>MVIDSKQDLPQYTKDSGSESDSDSSNNFIVESPSIPSSKSATVVLNSEEYEDDEGDDLNGLDAELIDNITYEGDEDETMFVGLKEKQKLHLSGVFRLQVVKGGIVYNNVHYNASREILTFWHPLSQSIPTIDFSHFAGWQDTFFMPRNNRFKIRDEEFKSFPCVLRVFNSNHTGLLEAGHLYRDVNYLWKPKEPYFPLNERTTYHLLHESDRIQSLSVPGYWSTPLEKLYLSHKNAAYDTRIMVIGGKNSGKSTFLRLLLEKFTQDIRDSTTSQEELVYLDLDPGQPEYSLPDSISLNKILSSPISLGQHLCQ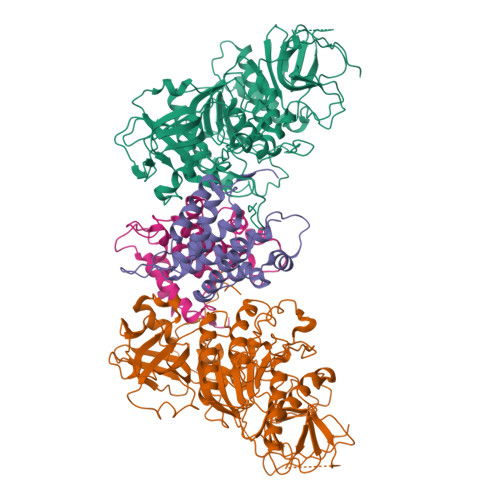GSNFQTLLQFYAGSSSPQDEPTSYLNCADKLIDHLEEQAFFGTSLLNLPGWIKGFGMQILNHIIRKYKPTHLLFLETANSKRHLDELTIPQSFSTSLRDAYAPEVVRVPAHSLNHTLSSRFHASQLRTFKILALFHKITQFDYDFAPLLKSAPLQISYGKGKSGIKGIQFPMEFQDLNPQDIKSALEGTVIGIYTYSGEDSLEVKSLNTFPILQSCTSSSKNFITLGLIHSIDTSQQIMNIYVPPCHTQILDKQPEDAQWIIVRNKTETPFCDFLPSPRTITWDDNIQIPFATFERRKKLEHVWKVRKNVMRRGQFMKR[2x];>[2x]MIPPRIVPWRDFAELEELKLWFYPKSKGTIEDKRQRAVQRVQSYRLKGSQYLPHVVDSTAQITCAVLLDEKEACLGVHQDSIPIRLSYVMALIRFVNGLLDPTQQSQFAIPLHTLAAKIGLPSWFVDLRHWGTHERDLPGLEMLRWAANEALSWLYDHYWNDEELEDDRDDDDDDDDTGYGYRRNDKLEKYMESLTKTLDKWKRLRNEFLEYKWVWENANDSLITSSNFSGDNLVNYDAEKRKSSHASSSETMIRENLRQWQELWKLSIYHNVVLEKFFNNYDPLLLKVLMLNLNNFDWKVIEWVARNYRTQQDDSNITTILKRKFNAWKELQKRLLDVIINNLNNKNFKNKWQNWEKLIDENASYLILYFCQSMLAKLETEKITGNSWRNKKRRKQIDSTVEIEAKLKENIDNLSLRFNEGEIKLYDFIPAEKDSVPLKKEVSPALKADTNDILGDLASLKQRMSSFGTVGKKNKQEENRATPVKNWSRVQNWKPKPFGVL> SRANDAPIVLLHGFTGWGREEMFGFKYWGGVRGDIEQWLNDNGYRTYTLAVGPLSSNWDRACEAYA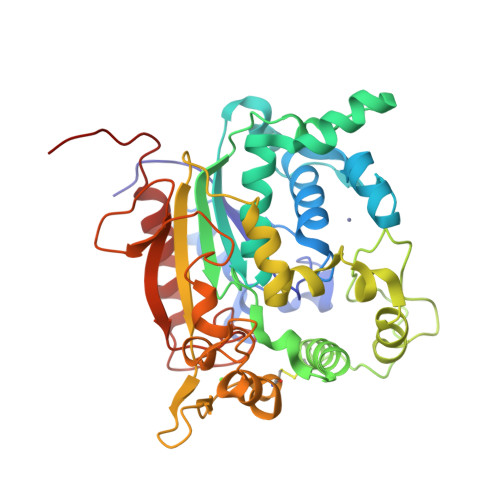QLVGGTVDYGAAHAAKHGHARFGRTYPGLLPELKRGGRIHIIAHSQGGQTARMLVSLLENGSQEEREYAKAHNVSLSPLFEGGHHFVLSVTTIATPHDGTTLVNMVDFTDRFFDLQKCVLKAAAVASNVPYTSQVYDFKLDQWGLRRQPGESFDQYFERLKRSPVWTSTDTARYDLSVPGAEKLNQWVKASPNTYYLSFATERTYRGALTGNYYPELGMNACSAVVCAPFLGSYRNATLGIDDRWLENDGIVNAFSMNGPKRGSTDRIVPYDGTIKKGVWNDMGTYNVDHLEVIGVDPNPLFDIRAFYLRLAEQLASLQPHHHHHH> MGSDKIHHHHHHLRINPGEITKVLEEKIKSFEEKIDLEDTGKVIQVGDGIARAYGLNKVMVSELVEFVETGVKGVAFNLEEDNVGIIILGEYKDIKEGHTVRRLKRIIEVPVGEELLGRVVNPLGEPLDGKGPINAKNFRPIEIKAPGVIYRKPVDTPLQTGIKAIDSMIPIGRGQRELIIGDRQTGKTAIAIDTIINQKGQGVYCIYVAIGQKKSAIARIIDKLRQYGAMEYTTVVVASASDPASLQYIAPYAGCAMGEYFAYSGRDALVVYDDLSKHAVAYRQLSLLMRRPPGREAYPGDIFYLHSRLLER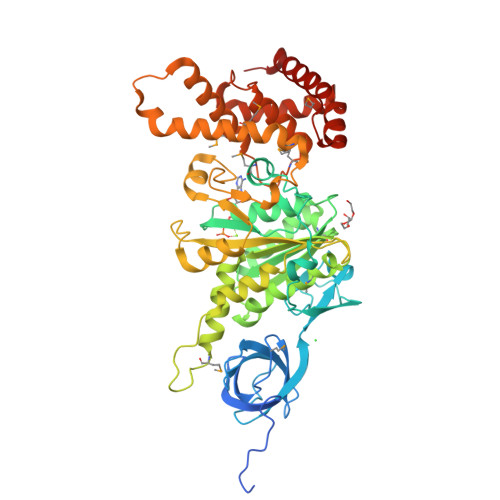AVRLNDKLGGGSLTALPIVETQANDISAYIPTNVISITDGQIYLEPGLFYAGQRPAINVGLSVSRVGGSAQIKAMKQVAGMLRIDLAQYRELETFAQFATELDPATRAQIIRGQRLMELLKQEQYSPMPVEEQVVVLFAGVRGYLDDLPVEEVRRFEKEFLRFMHEKHQDILDDIKTKKELTSETEEKLKKAIEEFKTTFRV>NDIGKTTTITRNKTSDGYTIITQNDKQIISYQSVDSSSKNEDGFTASIDARFIDDKYSS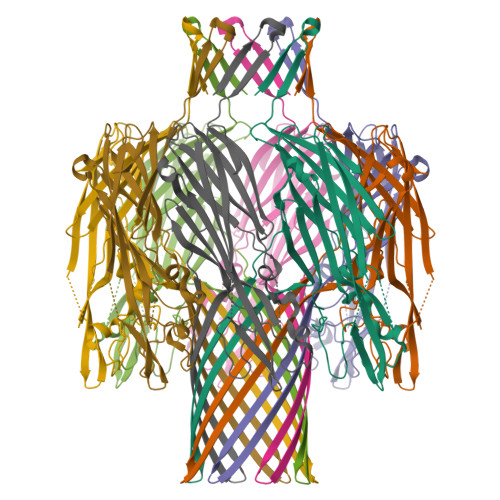EMTTLINLTGFMSSKKEDVIKKYNLHDVTNSTAINFPVRYSISILNESINENVKIVDSIPKNTISQKTVSNTMGYKIGGSIEIEENKPKASIESEYAESSTIEYVQPDFSTIQTDHSTSKASWDTKFTETTRGNYNLKSNNPVYGNEMFMYGRYTNVPATENIIPDYQMSKLITGGLNPNMSVVLTAPNGTEESIIKVKMERERNCYYLNWNGANWVGQVYSRLAFDTPNVDSHIFTFKINWLTHKVTAI[8x]>[2x]GPKSSDHVDLPYNLTATKIDSDVFVVTDRDFYSSNVLVAKMLDGTVVIVSSPFENLGTQTLMDWVAKTMKPKKVVAIN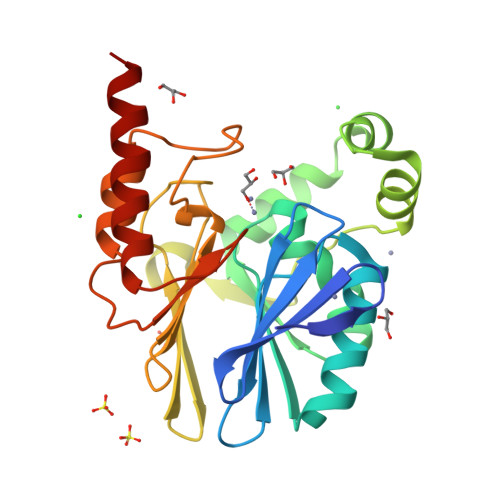THFHLDGTGGNEIYKKMGAETWSSDLTKQLRLEENKKDRIKAAEFYKNEDLKRRILSSHPVPADNVFDLKQGKVFSFSNELVEVSFPGPAHSPDNVVVYFPKKKLLFGGCMIKPKELGYLGDANVKAWPDSARRLKKFDAKIVIPGHGEWGGPEMVNKTIKVAEKAVGEMRL>ATRSPGVVISDDEPGYDLDLFCIPNHYAEDLERVFIPHGLIMDRTERLARDVMKEMGGHHIVALCVLKGGYKFFADLLDYIKALNRNSDRSIPMTVDFIRLKSYCNDQSTGDIKVIGGDDLSTLTGKNVLIVEDIIDTGKTMQTLLSLVRQYNPKMVKVASLLVKRTPRSVGYKPDFVGFEIPDKFVVGYALDYNEYFRDLNHVCVISETGKAKYKA[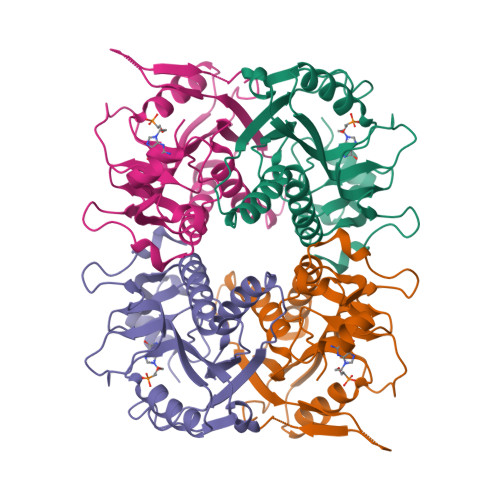2x]>[4x]MGHHHHHHSHMKGNIQQQIQLKSELASAEAKMEEQKQQLERHFEQSAN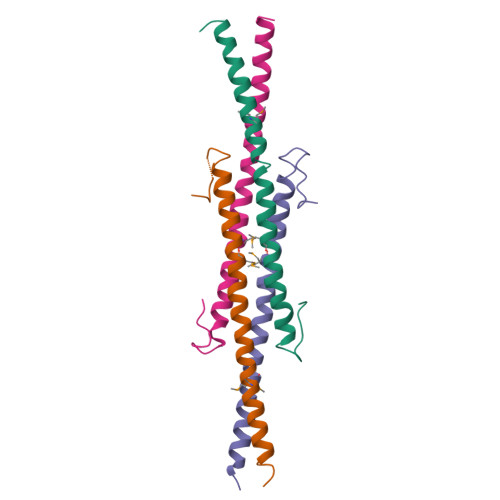LLENMAEDYKKLYTHFAQNSEQLLPESNQVEFFKRLKNHANGDEDNQPRDYSDGSSGLLKS>MTDLKASSLRALKLMHLATANDDDTDEKVIALCHQAKTPVGTTDAIYIYPRFIPIARKTLKEQGTPEIRIWTSTNFPHGNDDIDIALAETRAAIAYGADGVAVVFPYRALMAGNEQVGFDLVKACKEACAAANVLLSVIIETGELKDEALIRKASEISIKAGADHIVTSTGKVAVGATPESARIMMEVIRDMGVEKTVGFIPAGGVRTAEDAQKYLAIADELFGADWADARHYAFGASSLLASLLKALGHGDGKSASSYG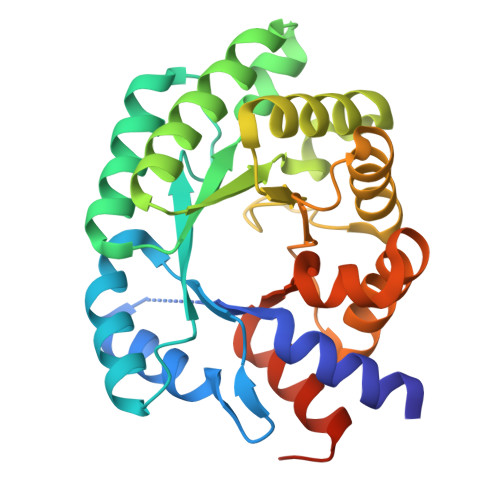SLE[2x]> SL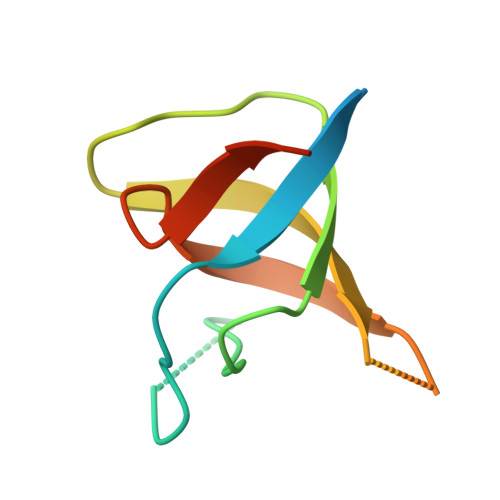DCMGDKSGKGGRLFVAVFDYETPDREGIIGFKAGDRFLIEEYAENGWCEAIHMDTAERPVQKGLVPGNFLRPLEGETKL> GSPNSMTGHHGWGY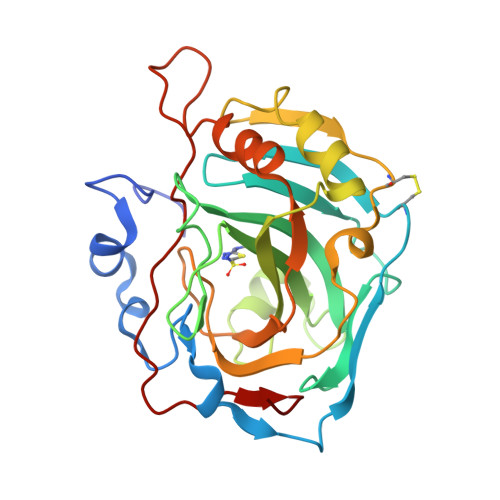GQDDGPSHWHKLYPIAQGDRQSPINIISSQAVYSPSLQPLELSYEACMSLSITNNGHSVQVDFNDSDDRTVVTGGPLEGPYRLKQFHFHWGKKHDVGSEHTVDGKSFPSELHLVHWNAKKYSTFGEAASAPDGLAVVGVFLETGDEHPSMNRLTDALYMVRFKGTKAQFSCFNPKSLLPASRHYWTYPGSLTTPPLSESVTWIVLREPISISERQMGKFRSLLFTSEDDERIHMVNNFRPPQPLKGRVVKASFRA> MGKKITILLGALLPFTSAVADEPALSPEAITSAQVFSTQSKETYTYVRCWYRTGNSHDESATDWEWAENPDGSYFTIDGYWWSSVRLKNMFYTNTSQNVIKQRCEETLGVTHDAADITYFAADNRWSYNHTIWTNDPVMQADQINKIVAFGDSLSDTGNIFNAAQWRFPNPDTWFLGHFS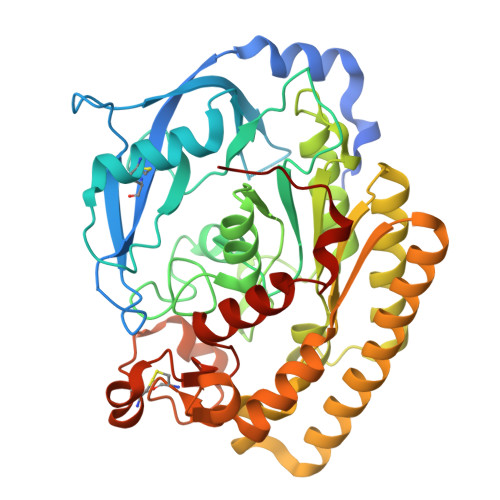NGFVWTEYIAQAKKLPLYNWAVGGAAGSNQYVALTGVKDQVLSYLTYAKMAKNYKPENTLFTLEFGLNDFMNYNREVVDVKTDFSTALIKLTDAGAKNIMLMTLPDATKAPQFKYSTQAEIEKVRAKIVEFNEFIKAQAAFYIIQGYNITLYDTHGLFEQLTQNPQQHGFVNASDACLNINRASSADYLYSHSLTNECATHSSDKYVFWDVTHPTTAVHKYIAEKMLAPGAGMQRFNFHHHHHH N-[3-methyl-4-({3-[2-(methylamino)pyrimidin-4-yl]pyridin-2-yl}oxy)naphthalen-1-yl]-1H-benzimidazol-2-amine | C28 H23 N7 O | 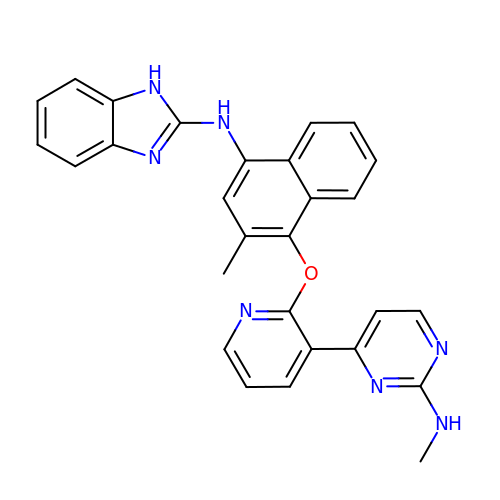JXKDTYDBDDKIPY-UHFFFAOYSA-N> AKTEPSEKSVEIMRKFSEQYARRSGTYFCVDKGVTSVVIKGLAEHKDS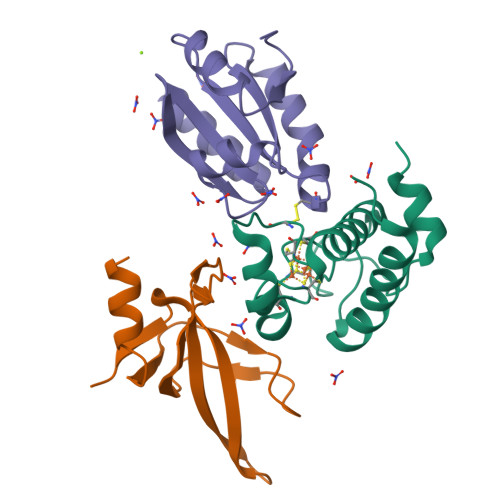YGAPLCPCRHYDDKAAEVGQGFWNCPCVPMRERKECHCMLFLTPDNDFAGKDQTITSDEIKETTANM;> DIAVKSAASVDADADLSSSTSLETEEDEKAKEKIGARVRVTVPLKVYHVVRVPEVELMGMEGFIKDYVVLWKGKKISANLPFKVQFVKEIEGRGPVKFFTHLKEDEFELIDP;> ETVNVTVGQVTEVDKDTFWPIVKAAGDKIVVLDMYTQWCGPSKVIAPKYKELSEKYQDMVFLKLDCNQDNKPLAKELGIRVVPTFKILKDNKVVKEVTGAKYEDLLAAIEAARSG>GSMATSTSTSTPIIFYDIAQRPPVAETCCAVNPWKSRLALNFKAVPYTTTWVKMPDISSVRASLNVPACRKFADGSDFNTLPIIHDPATDSLIGDSLDIAAYLQRTYPASGAGDLFPPQKLDYAVGRDMQQLLFPLSEIRASPELADYARFNSNVDAAFTAHVGLMVHGLPLDPATADVTKAEFVRRAGLSSWDDLEMVGEARDKMMQSLRNMLGDLAALFRKDASGPFLLGQRATYADMIVGGWLRMMRATLPVSEWQEARACHGAIFGQLHDALDKYAE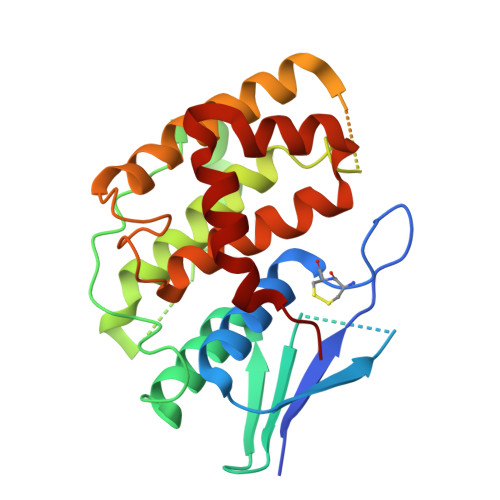VK[2x]>MEKRMSTQQRAAGNACPTAAFSFDPARLAQRRRWAGAFAALCGLALSPSALLAEEHSQHQDHAVELAPSVVTGVAQSSPLTIVTNPKEPRQPVPASDGADYLKTIPGFAVIRNGGSNGDPVLRGMFGSRLNILTNGGMMLGAAPNRADAPTSYISPETYDKLTVIKGPQTVLWGPGASAGTILFEREPERFGELGSRVNASLLAGSNGRFDKVLDAAAGNRLGYLRFTGNHAQSDDYEDGAGNTVPSRWKKWNGDVAVGWTPDEDTLIELTAGKGDGEARYAGRGMDGSQFKRESLGLRFVKSNVSDVLEKVEAQVYYNYADHIMDNFRLRTPDPSSMMPMPMASQVDRRTLGGRLAATWRWDDFKLVTGVDAMRNEHRARGSKYDMMTDYYTDADQFPWSKDAVFHNYGAFGELTWFAAERDRLIGGLRLDRASVKDYRQTLKSGHMGHAMANPTANDTRADTLPSGFVRYEHDLADSPTTLYAGLGHAERFPDYWELFSPKRGPNGSVNAFDKIKPEKTTQLDFGLQYNGDKLQAWASGYVGVVQDFILFSYREGMMGSSTQATNVD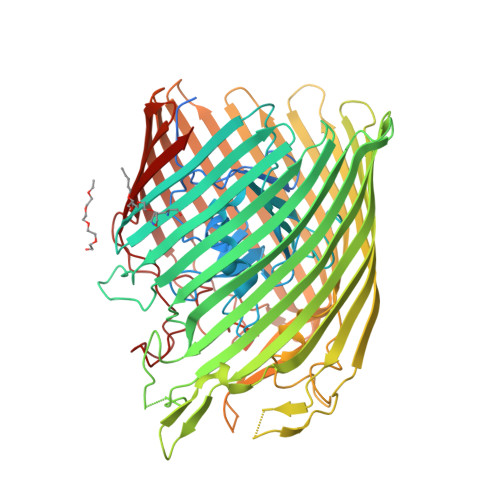ARIMGGELGASYQLTGNWKTDASLAYAWGKNSSDDRALPQIPPLEARFGLTYEEGDWSAGSLWRVVAPQNRIARDQGNVVGKDFDKSAGFGVFSLNGAYRVTRNVKLSAGVDNLFDKDYTEHLNKAGDAGFGFSANETVPEPGRTFWTKVDFSF[2x]> GKITLYEDRGFQGRHYECSSDHPNLQPYLSRC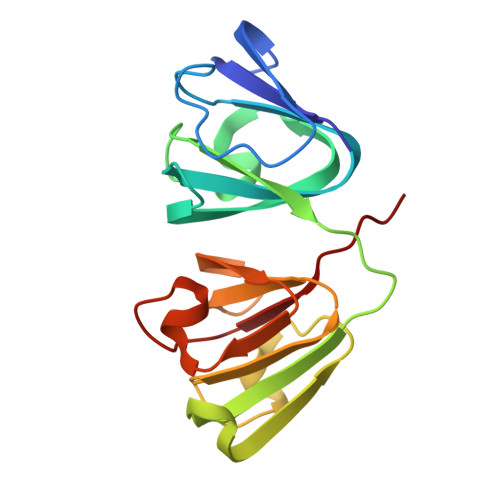NSARVDSGCWMLYEQPNYSGLQYFLRRGDYADHQQWMGLSDSVRSCRLIPHSGSHRIRLYEREDYRGQMIEFTEDCSCLQDRFRFNEIHSLNVLEGSWVLYELSNYRGRQYLLMPGDYRRYQDWGATNARVGSLRRVIDFS> GDDLEVGKNIDESAYSGIYENNAYLRDGKSNLVSKVVELHGETYATTVKMGLSKTPNTATSAKVKIDAAYLETYNKAHNTDFALYPQDLVTFANEGILTVNANTKSAEVEMTIRAGEGLQEDKTYAIPVAISDQSSDITIKDEDAKHCIYLVKDMRNAGDAYKGEGVMQGYLFFEVNDVNPLNTLSFQLENGKLLWDVVVLFAANINYDAEAGRPRVQCNPNVQYLLDNNETLLQPLRRRGVKVLLGLLGNHDITGLAQLSEQGAKDFAREVAQYCKAYNLDGVNYADLYSNSPDLSNPSLTNPST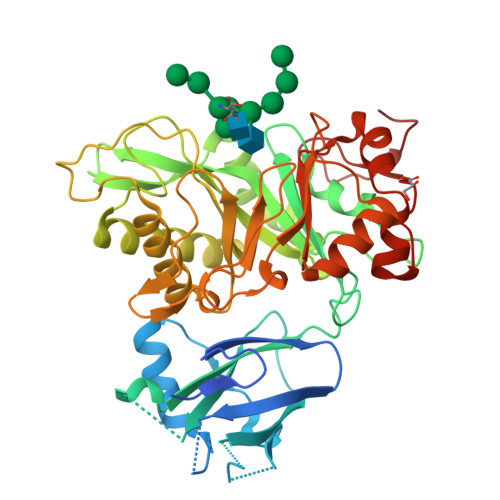AAAARLCYETKQAMPDKLVTVFDWGQMYGVATVDGVDAKEWIDIVVANYGSAAYPIGQMTKKQCSGISMEFNLGGGGSLSASKAQSMIDGGYGWFMGFAPSPAKYGSVFSRLQGGGEVLYGSNVAAPTIFYKKNDPTPYKYPDDL>GSMEEEAETEEQQRFSYQQRLKAAVHYTVGCLCEEVALDKEMQFSKQTIAAISELTFRQCENFAKDLEMFARHAKRTTINTEDVKLLARRSNSLLKYITDKSEEIAQINLER[6x];>GSMEGAGAGSGFRKELVSRLLHLHFKDDKTKVSGDALQLMVELLKVFVVEAAVRGVRQAQAEDALRVDVDQLEKVLPQLLLDF[6x];>GAMDPMRQSSLKKDWFLSEEEFKLWNRLYRLRDSDEIKEITLPQVQFSSLQNEENKPAQESTTGIHQLSLSEWRLWQDHPLPTHQV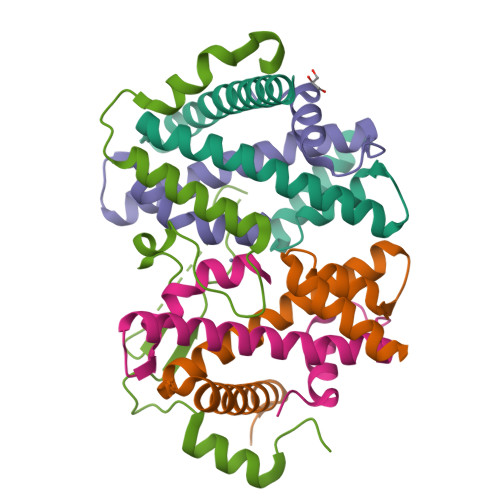DHSDRCRHFIGLMQMIEGMRHEEGECSYELEVESYLQMEDVTSTFIAPRNE[3x]> SLSAAQKDNVKSSWAKASAAWGTAGPEFFMALFDAHDDVFAKFSGLFSGAAKGTVKNTPEMAAQAQSFKGLV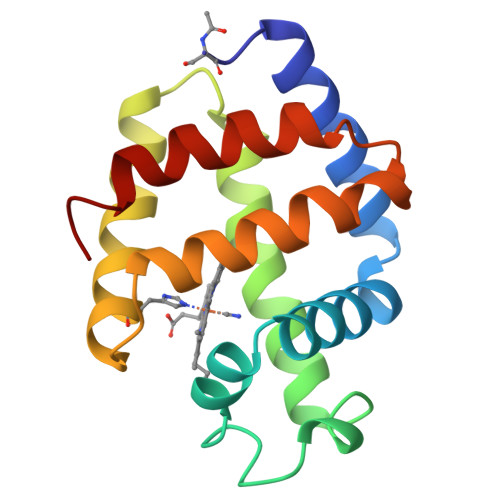SNWVDNLDNAGALEGQCKTFAANHKARGISAGQLEAAFKVLAGFMKSYGGDEGAWTAVAGALMGMIRPDM>MDYKDDDDKAVFSKLQLLGQAIPPKQYAPGVVGMLAVFALIKLYKQDIRGTKHLVAKTKEGKKERAVVDKVFFSRLIQILKIMVPRTFCKETGYLVLIAVMLVSRTYCDVWMIQNGTLIESGIIGRSRKDFKRYLLNFIAAMPLISLVNNFLKYGLNELKLCFRVRLTKYLYEEYLQAFTYYKMGNLDNRIANPDQLLTQDVEKFCNSVVDLYSNLSKPFLDIVLYIFKLTSAIGAQGPASMMAYLVVSGLFLTRLRRPIGKMTITEQKYEGEYRYVNSRLITNSEEIAFYNGNKREKQTVHSVFRKLVEHLHNFILFRFSMGFIDSIIAKYLATVVGYLVVSRPFLDLSHPRHLKSTHSELLEDYYQSGRMLLRMSQALGRIVLAGREMTRLAGFTARITELMQVLKDLNHGKYERTMVSQQEKGIEGVQVIPLIPGAGEIIIADNIIKFDHVPLATPNGDVLIRDLNFEVRSGANVLICGPNGCGKSSLFRVLGELWPLFGGRLTKPERGKLFYVPQRPYMTLGTLRDQVIYPDGREDQKRKGISDLVLKEYLDNVQLGHILEREGGWDSVQDWMDVLSGGEKQRMAMARLFYHKPQFAILDQCTSAVSVDVEGYIYSHCRKVGITLFTVSHRKSLWKHHEYYLHMDGRGNYEFKQITEDTVEFGS[2x]

Human ABC transporters ABCD1–3 are all localized on the peroxisomal membrane and participate in the β-oxidation of fatty acyl-CoAs, but they differ from each other in substrate specificity. The transport of branched-chain fatty acids from cytosol to peroxisome is specifically driven by ABCD3, dysfunction of which causes severe liver diseases such as hepatosplenomegaly. The overall structure exhibits a two-fold symmetric homodimer, with each subunit containing a nucleotide-binding domain (NBD) and a transmembrane domain (TMD). The helices TM4 and TM5 from one TMD are swapped to the opposite TMD, i.e., domain swapping, which is a typical feature of type-IV ABC transporters.

In order to capture the substrate release state of ABCD3, we prepared the cryo-EM sample with ABCD3 E596Q mutant via adding 10 mM ATP/Mg2+ and 0.5 mM phytanoyl-CoA, and solved an ATP-bound ABCD3 structure at a resolution of 3.2 Å with C2 symmetry. In this structure, the two NBDs dimerize in a “head-to-tail” mode. At the interface of two NBDs, two ATP molecules are sandwiched by the Walker A motif from one NBD and the ABC signature motif from the other. In consequence, the conformational changes in NBDs are transferred to TMDs via two pairs of coupling helices, and eventually make the ATP-bound ABCD3 exhibit an outward-facing conformation. The two TMDs pack against each other at the cytosol side, while separating at the peroxisomal matrix side, forming a narrow transport cavity to peroxisome. When comparing the ATP- and phytanoyl-CoA-bound ABCD3 structures, the ATP-bound structure displays a scissor-like movement, resulting in an enlarged exit of the translocation cavity. Specifically, TM4 and TM5 are split into two short helices due to the conformational changes, and the first half (lower half in Fig. 4b) moves towards the translocation cavity by ~13.7 Å as measured by the I273 Cα atoms. Although phytanoyl-CoA was added during sample preparation for the structure analysis of ATP-bound ABCD3, we did not observe clear density for the full-length substrate, but a pair of extra densities in the translocation cavity. Based on the density shapes, they could be tentatively fitted with a pair of CoA molecules located symmetrically in a positively charged pocket, except the missing cysteamine group. Compared to the phytanoyl-CoA-bound ABCD3, the binding site of CoA is localized deeper towards the cytosol.>[2x]GMASLPKRIIKETEKLVSD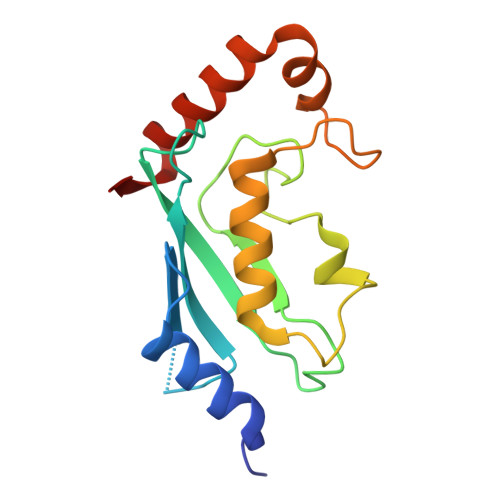PVPGITAEPHDDNLRYFQVTIEGPEQSPYEDGIFELELYLPDDYPMEAPKVRFLTKIYHPNIDRLGRIELDVLKTNWSPALQIRTVLLSIQALLASPNPNDPLANDVAEDWIKNEQGAKAKAREWTKLYAKKKPE>GELLDPCGYISPESPVVQLHSNFTAVCVLKEKCMDYFHVNANYIVWKTNHFTIPKEQYTIINRTASSVTFTDIASLNIQLTCNILTFGQLEQNVYGITIISGLPPEKPKNLSCIVNEGKKMRCEWDGGRETHLETNFTLKSEWATHKFADCKAKRDTPTSCTVDYSTVYFVNIEVWVEAENALGKVTSDHINFDPVYKVKPNPPHNLSVINSEELSSILKLTWTNPSIKSVIILKYNIQYRTKDASTWSQIPPEDTASTRSSFTVQDLKPFTEYVFRIRCMKEDGKGYWSDWSEEASGITYEDRPSKAPSFWYKIDPSHTQGYRTVQLVWKTLPPFEANGKILDYEVTLTRWKSHLQNYTVNATKLTVNLTNDRYLATLTVRNLVGKSDAAVLTIPACDFQATHPVMDLKAFPKDNMLWVEWTTPRESVKKYILEWCVLSDKAPCITDWQQEDGTVHRTYLRGNLAESKCYLITVTPVYADGPGSPESIKAYLKQAPPSKGPTVRTKKVGKNEAVLEWDQLPVDVQNGFIRNYTIFYRTIIGNETAVNVDSSHTEYTLSSLTSDTLYMVRMAAYTDEGGKDGPEFTFTTPK[2x];>GSPDPRAELDSTVLLTRSLLADTRQLAAQLRDKFPADGDHNLDSLPTLAMSAGALGALQLPGVLTRLRADLLSYLRHVQWLRRAGGSSLKTLEPELGTLQARLDRLLRRLQLLMSRLALPQPPPDPPAPPLAPPSSAWGGIRAAHAILGGLHLTLDWAVRGLLLLKTRL[2x];>GSSPCPQAWGPPGVQYGQPGRSVKLCCPGVTAGDPVSWFRDGEPKLLQGPDSGLGHELVLAQADSTDEGTYICQTLDGALGGTVTLQLGYPPARPVVSCQAADYENFSCTWSPSQISGLPTRYLTSYRKKTVLGADSQRRSPSTGPWPCPQDPLGAARCVVHGAEFWSQYRINVTEVNPLGASTRLLDVSLQSILRPDPPQGLRVESVPGYPRRLRASWTYPASWPSQPHFLLKFRLQYRPAQHPAWSTVEPAGLEEVITDAVAGLPHAVRVSARDFLDAGTWSTWSPEAWGTPSTGT[2x]

Interleukin (IL-), an IL-6 family cytokine, has pivotal roles in autoimmune diseases, fibrotic complications, and solid cancers. IL-11 activates downstream signalling pathways by binding its two cell surface receptors: the IL-11 specific receptor, IL-11Rα, and the signal-transducing receptor, glycoprotein (gp)13013,26. Following the formation of the receptor complex, the Janus kinase (JAK)/signal transducer and activator of stat (STAT) and extracellular signal regulated kinase (ERK)/mitogen-activated protein kinase (MAPK) pathways are primarily activated. IL-11 and IL-6 utilise a homodimer of gp13026,34,35 while other IL-6 family members exploit a heterodimer of gp130 with a second signal-transducing receptor, such as LIF receptor (LIFR), OSM receptor (OSMR), IL-27R/WSX-1 or IL-12 receptor β−2 subunit (IL-12Rβ2).

To understand the molecular mechanisms underpinning human IL-11 signalling complex formation, we solved three structures of the complex containing either the cytokine binding domains of gp130 (gp130D1-D3) or the complete extracellular domains of gp130 (gp130EC) using electron cryo-microscopy (cryo-EM) and X-ray crystallography. We obtained a 3.5 Å resolution cryo-EM reconstruction of the IL-11Δ10/IL-11RαD1-D3/gp130D1-D3 complex (referred to as the gp130D1-D3 complex), and a 3.8 Å resolution cryo-EM reconstruction of the IL-11Δ10/IL-11RαD1-D3/gp130EC complex (referred to as the gp130EC complex). D1 of IL-11Rα was not visible in the gp130D1-D3 complex map and was poorly defined in the gp130EC complex map, suggesting this domain is flexible. D5-D6 of gp130 were poorly defined in the gp130EC complex density and were not included in the deposited model. We considered the possibility that structural dynamics of gp130 D4-D6 contributed to the decreasing density quality with distance from the cytokine binding regions. Histograms of the distributions along each trajectory are unimodal, indicating continuous motion. This analysis shows that the D4-D6 region of gp130 is dynamic and is not stabilised upon complex formation. A multistate model, allowing flexibility of gp130 domains D4-D6 and IL-11Rα D1, fit the SAXS data for the gp130EC complex better than our single consensus model of the complex, further supporting flexibility of these domains within the complex. The affinity of the IL-11RαD1-D3/IL-11Δ10 binary complex for gp130EC, (KD 4 ± 2 nM, ΔH -20 ± 1 kJ/mol; Fig. 2Iiii) is very similar to the affinity for gp130D1-D3, indicating that the membrane-proximal (D4-D6) domains of gp130 do not contribute substantially to complex formation. The observation that D4-D6 of gp130 are flexible with respect to the membrane distal domains (D1-D3) provides information on the potential relative positions of the two D6 domains within the complex that may affect positioning of the transmembrane and cytoplasmic domains.>[2x]AGLPVIMCLKSNNHQKYLRYQSDNIQQYGLLQFSADKILDPLAQFEVEPSKTYDGLVHIKSRYTNKYLVRWSPNHYWITASANEPDENKSNWACTLFKPLYVEEGNMKKVRLLHVQLGHYTQNYTVGGSFVSYLFAESSQIDTGSKDVFHVIDWKSIFQFPKGYVTFKGNNGKYLGVITINQL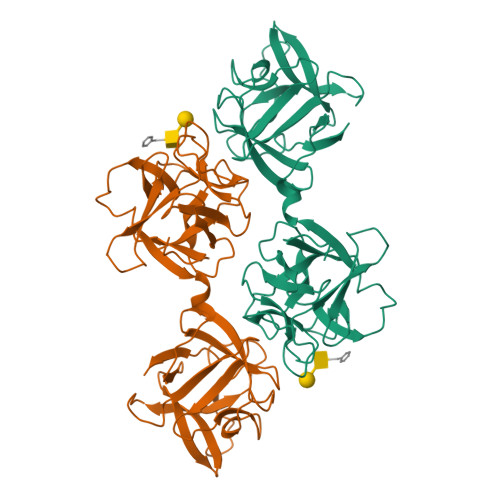PCLQFGYDNLNDPKVAHQMFVTSNGTICIKSNYMNKFWRLSTDDWILVDGNDPRETNEAAALFRSDVHDFNVISLLNMQKTWFIKRFTSGKPGFINCMNAATQNVDETAILEIIELGQNN>GGUGGCUGUU[5x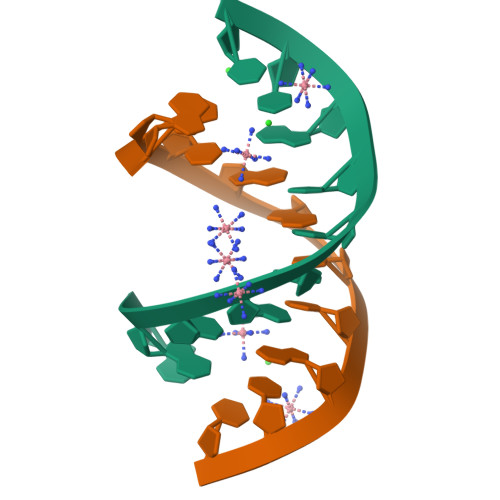]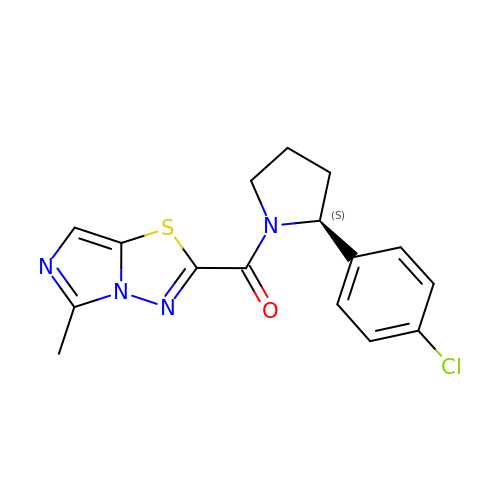[(2S)-2-(4-chlorophenyl)pyrrolidin-1-yl](5-methylimidazo[5,1-b][1,3,4]thiadiazol-2-yl)methanone | C16 H15 Cl N4 O S | SAVNWXMDAMFANR-ZDUSSCGKSA-N> MRCIGMSNRDFVEGVSGGSWVDIVLEHGSCVTTMAKNKPTLDFELIKTEAKQPATLRKYCIEAKLTNTTTESRCPTQGEPSLNEEQDKRFVCKHSMVDRGWGNGCGLFGKGGIVTCAMFRCKKNMEGKVVQPENLEYTIVITPHSGEEHAVGNDTGKHGKEIKITPQSSITEAELTGYGTVTMECSPRTGLDFNEMVLLQMENKAWLVHRQWFLDLPLPWLPGADTQGSNWIQKETLVTFKNPHAKKQDVVVLGSQEGAMHTALTGATEIQMSSGNLLFTGHLKCRLRMDKLQLKGMSYSMCTGKFKVVKEIAETQHGTIVIRVQYEGDGSPCKIPFEIMDLEKRHVLGRLITVNPIVTEKDSPVNIEAEPPFGDSY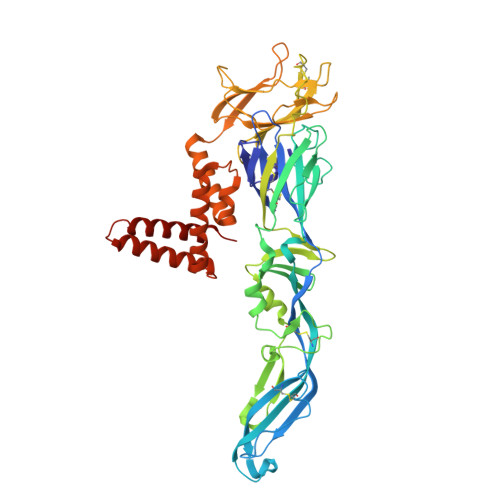IIIGVEPGQLKLNWFKKGSSIGQMFETTMRGAKRMAILGDTAWDFGSLGGVFTSIGKALHQVFGAIYGAAFSGVSWTMKILIGVIITWIGMNSRSTSLSVTLVLVGIVTLYLGVMVQA>MSDVQSSLTGTWYNELNSKMELTANKDGTLTGKYLSKVGDVYVPYPLSGRYNLQPPAGQGVALGWAVSWENSKIHSATTWSGQFFSESSPVILTQWLLSSSTARGDVWESTLVGNDSF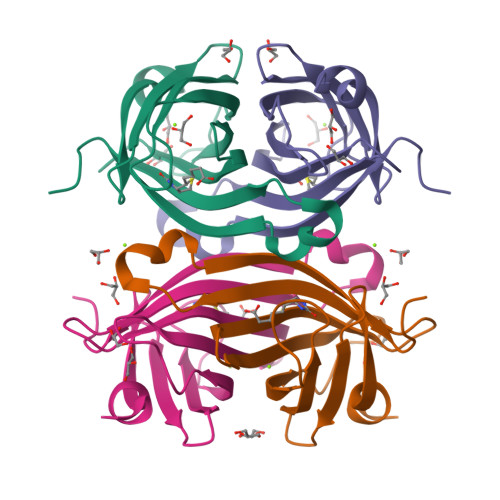TKTAPTEQQIAHAQLHCRAPRLK[2x]>HAHLKSATPAADSTVAAPADLRLTFSEGVEATFTKVSLSKDGTEVAIKGLETPDADKKTLVVTPAAPLAAGNYKVVWNAVSVNTHKSNGEYSF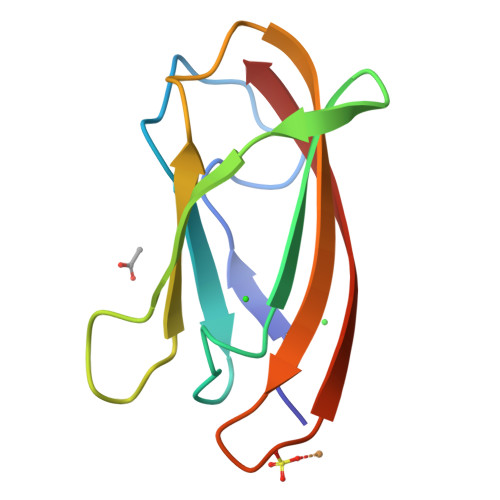KVGQ[2x]>[2x]MSHMNLVVYAQRGASMPYTRYDTDDAARGGGATLQSAPNFDQALTASEASGQRYIALPSNGSYAQWTIRPGEGGDGVTMRFTMPDSANGMGLNGSLDVYVNGVKAKTVPLTSYYSWQYFSSDHPADTPAGGRPLFRFDEVHWKMDTPLQPGDTIRIQKSGADSLEYGVDFLEIEAVPAAIARPANSVSVTDFGAVANDGQDDLAAFEAAVNAAVTSGKILYIPAGTFHLGNMWKIGSVANKINNITIMGAG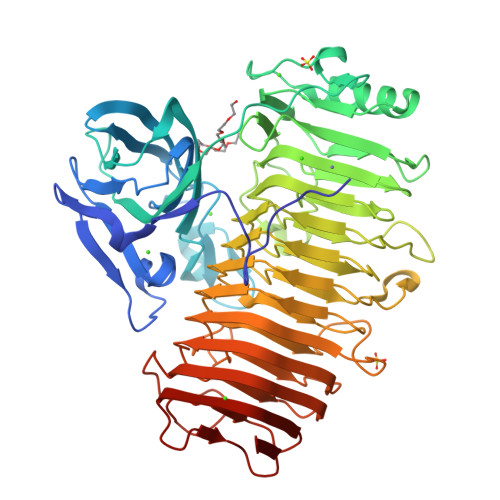IWHTNIQFTNPNQASGGISFRVTGQLDFSHIYMNSNLRSRYGEQAVYKGFMDNFGTNSKVHNVWVEHFECGFWVGDYAHTPAIIANGLVIENSRIRNNLADGVNFAQGTSNSTVRNSSIRNNGDDGLAVWTSNVNGAPAGVNNTFSYNTIENNWRAAGIAFFGGSGHKATHNLIVDTVGGSAIRMNTVFPGYHFQNNTGIVFSDTTIINSGTSRDLYNGERGAIDLEASNDPIKNVTFTNIDIINTQRSAIQFGYGGGFENIVFNNININGAGKDGVLTSRFSSPHPGAAIYTYTGNGSATFNNLTTNDIAHPNLYFIQNGFNLTIQ>[5x]GSSEHLKREHSLIKPYQGVGSSSMPLWDFQGSTILTSQYVRLTPDERSKEGSIWNHQPCFLKDWEMHVHFKVHGTGKKNLHGDGIALWYTRD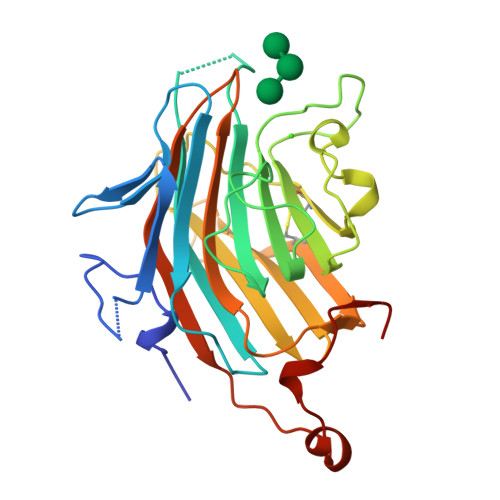RLVPGPVFGSKDNFHGLAIFLDTYPNDETTERVFPYISVMVNNGSLSYDHSKDGRWTELAGCTADFRNRDHDTFLAVRYSRGRLTVMTDLEDKNEWKNCIDITGVRLPTGYYFGASAGTGDLSDNHDIISMKLFQLMVEHTPDEENIDWTKIEPSVNFLKS>[2x]MGSSHHHHHHSQDPNSMPDNTIQWDKDADGIVTLTMDDPSGSTNVMNEAYIESMGKAVDRLVAEKDSITGVVVASAKKTFFAGGDVKTMIQARPEDAGDVFNTVETIKRQLRTLETLGKPVVAAINGAALGGGLEIALACHHRIAADVKGSQLGLPAVTLGLLPGGGGVTRTVRMFGIQNAFVSVLAQGTRFKPAKAKEIGLVDELVATVEELVPAAKAWIKEELKANPDGAGVQPWDKKGYKMPGGTPSSPGLAAILPSFPSNLRKQLKGAPMPAPRAILAAAVEGAQVDFDTASRIESRYFASLVTGQVAKNMMQAFFFDLQAINAGGSRPEGIGKTPIKRIGVLGAGMMGAGIAYVSAKAGYEVVLKDVSLEAAAKGKGYSEKLEAKALERGRTTQERSDALLARITPTADAADFKGVDFVIEAVFENQELKHKVFGEIEDIVEPNAILGSNTSTLPITGLATGVKRQEDFIGIHFFSPVDKMPLVEIIKGEKTSDEALARVFDYTLAIGKTPIVVNDSRGFFTSRVIGTFVNEALAMLGEGVEPASIEQAGSQAGYPAPPLQLSDELNLELMHKIAVATRKGVEDAGGTYQPHPAEAVVEKMIELGRSGRLKGAGFYEYADGKRSGLWPGLRETFKSGSSQPPLQDMIDRMLFAEALETQKCLDEGVLTSTADANIGSIMGIGFPPWTGGSAQFIVGYSGPAGTGKAAFVARARELAAAYGDRFLPPE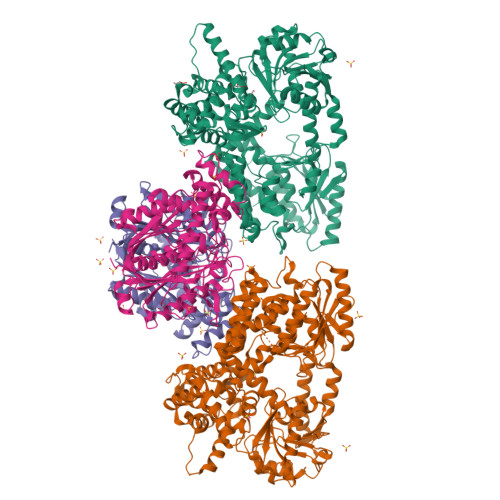SLLS;>[2x]MSEEAFIYEAIRTPRGKQKNGSLHEVKPLSLVVGLIDELRKRHPDLDENLISDVILGCVSPVGDQGGDIARAAVLASGMPVTSGGVQLNRFAASGLEAVNTAAQKVRSGWDDLVLAGGVESMSRVPMGSDGGAMGLDPATNYDVMFVPQSIGADLIATIEGFSREDVDAYALRSQQKAAEAWSGGYFAKSVVPVRDQNGLLILDHDEHMRPDTTKEGLAKLKPAFEGLAALGGFDDVALQKYHWVEKINHVHTGGNSSGIVDGAALVMIGSAAAGKLQGLTPRARIVATATSGADPVIMLTGPTPATRKVLDRAGLTVDDIDLFELNEAFASVVLKFQKDLNIPDEKLNVNGGAIAMGHPLGATGAMILGTMVDELERRNARRALITLCIGGGMGVATIIERV> MAKHATPKLDQLESGPWPSFVSDIKQEAAYRAANPKGLDYQVPVDCPEDLLGVLELSYDEGETHWKHGGIVGVFGYGGGVIGRYCDQPEKFPGVAHFHTVRVAQPSGKYYSADYLRQLCDIWDLRGSGLTNMHGSTGDIVLLGTQTPQLEEIFFELTHNLNTDLGGSGSNLRTPESCLGKSRCEFACYDSQAACYELTMEYQDELHRPAFPYKFKFKFDACPNGCVASIARSDFSVIGTWKDDIKIDAEAVKAYVAGEFKPNAGAHSGRDWGKFDIEAEVVNRCPSKCMKWDGSKLSIDNKECVRCMHCINTMPRALHIGDERGASILCGAKAPILDGAQMGSLLVPFVAAEEP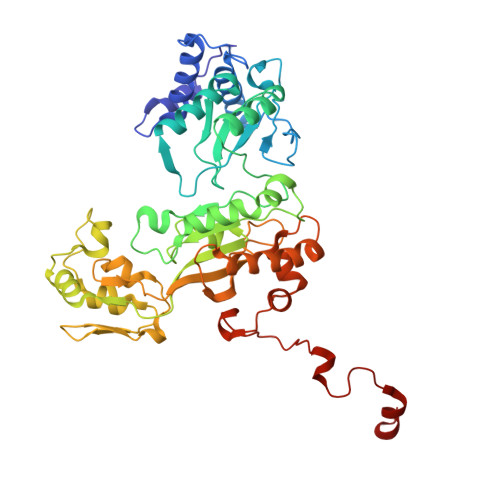FDEIKEVVEKIWDWWMEEGKNRERLGETMKRLSFQKLLEVTEIAPVPQHVKEPRTNPYIFFKEEEVPGGWDRDITEYRKRHLR One of these energy-consuming enzymes is the conserved huge AAA+-type ATPase Rea1 (also known as Mdn1), which is composed of a hexameric AAA+-ATPase domain, followed by a long tail consisting of an α-helical linker region, a flexible aspartate/glutamate (D/E)-rich domain and a C-terminal metal-ion-dependent adhesion site (MIDAS) homologous to the inserted (I) domain within the α-subunits (αI) of integrins that mediate ligand recognition. The conserved interaction between the C-terminal Rea1-MIDAS and the Rsa4-UBL (ubiquitin-like domain) or Ytm1-UBL is essential for assembly of the 60S pre-ribosome in a reaction mediated by the Rea1 ATPase upon ATP hydrolysis that leads to the removal of Ytm1 and Rsa4 from distinct pre-60S intermediates. In this study, we report crystal structures of the Chaetomium thermophilum (Ct) Rea1-MIDAS, both alone and in complex with its pre-ribosomal substrates, the CtYtm1- or CtRsa4-UBL domains. Besides displaying the typical MIDAS fold known for integrins, the CtRea1-MIDAS crystal structures reveal evolutionary conserved Rea1 specific structural elements.

Next, we aimed to structurally investigate the complex between CtRea1-MIDAS and its two ligands, the ubiquitin-like domains (UBL) of CtRsa4 and CtYtm1. However, purification and crystallization proved to be challenging and might have been impeded by the conserved but flexible MIDAS loop (element II). Since this loop (deletion of amino acids 4734–4773 in CtRea1, or 4657–4696 in ScRea1) is dispensable for MIDAS–Rsa4 interaction, we replaced it with a short Gly-Ser-Gly linker. Using these trimmed constructs, we were able to reconstitute the complexes CtRea1-MIDAS∆loop–CtRsa4-UBL and CtRea1-MIDAS∆loop–CtYtm1-UBL, which readily crystallized, allowing us to solve their crystal structures at 1.89 and 1.84 Å, respectively. Although the overall structures of the Rea1-MIDAS ∆loop domain in complex with either Rsa4-UBL or Ytm1-UBL are highly similar to the MIDAS apo structure, the terminal helices α1 and α9 were slightly tilted (as observed upon binding of integrins to its ligands for the C-terminal helix). The Mg2+-binding site in this case is fully ordered and the metal ion is coordinated cooperatively by the MIDAS and UBL domains. However, one unforeseen major structural re-arrangement concerns the Rea1-specific element III, which in the apo structure forms a loop that crawls along helices α1 and α9 and was not fully resolved, but in the ligand-bound form becomes re-arranged, the short helix α8 partially unfolds and forms a β-hairpin that provides an additional binding site for the UBL domains of Rsa4 and Ytm1. To investigate the importance of this binding site for interaction with the ligand Rsa4, we mutated two residues (CtRea1 F4951 > A/R; CtRea1 I4959 > A/R), which lie within the β-hairpin and directly contact the Rsa4- or Ytm1-UBL.

> MHISDEQLKRPLRDYGEALEMWSTFQTKTQALSQSLSSQLRLILTGSGIPSKRAYQILLCVDDSSSMSDDNRSTAGNLALESLVMVARALTVLEAGQIGVMGFGTDVFVAHALTDPPFTSQDAGARVLQQFTFRQDSTDMVLLLRRTIDHFREARLIQASSSRGGEDLWQLALILSDGLVQSRDHARLRPLLREAMEQRVMVVFIVMDDARSRKGHSVLELKEARFGPDGVPVIHRYLDSFPFPYYLIVHHLEDLPGALAALLRTWFAEVNSGSHHHHHH;> MKHHHHHHPMATDLGSFKANFIDSDGNQMTDVVEINFADATEKNISNLLNTLLGRDREEFTPYRFRIHIPGKDLIIDQYPNDLLSLLQKHGVTNPFETTITLSAEPQA>[2x]MDLKIKNKVCIITGGAKGIGYGIAKLWASEGGIPVIFSRSMPKEHDKELKKLSSEYEFYEIDLKNYEQIEKLVKKVAIKHGGIYALVNNAGTNDNLHIENTSTQDLIKSYENNLFHYYTMTKECLPYIKKEQGSILNIVSKTGITGQGRTSAYASAKAAQMGFTREWACAFAKDNVRVNAIAPAEVMTPLYEKWLQNFPNPKEQYEKIAKAIPLGHRFTTIEEIANTAVFTLSPLASHTTGQILMPDGGYVHLDRALNWDENTRGHHHHHH

We also characterize the putative dehydrogenase Cj0485 through crystallography, enzymology, and multiple biological assays to confirm its function as a fucose dehydrogenase, which we have named FucX. Several aldose sugars in both d- and l-configurations were screened as substrates and Cj0485 displayed substantial activity on l-fucose and d-arabinose and with low levels of activity on l-galactose. The Cj0485 monomer adopts a Rossmann-like fold comprising a central seven-stranded twisted β-sheet sandwiched between two trios of parallel α-helices. The holo-enzyme’s asymmetric unit contained four monomers that were arranged as tetramers with identical D2 symmetry to the crystallographic tetramer observed in the apo-complex. PISA31 analysis predicts this recurring tetramer to be a stable conformation, supporting the likelihood that the tetramer is the biologically relevant assembly of the enzyme.

To provide insight into the substrate specificity of Cj0485, we solved X-ray crystal structures of this enzyme alone and in complex with NADP+. The apo-enzyme crystallized in the space group C2221 with two monomers in the asymmetric unit and the crystallographic lattice generates a tetramer with D2 symmetry. A Cj0485 monomer from the apo-structure superimposes on an apo-FabG monomer with a root-mean-square-deviation (RMSD) of 0.9 Å (over 246 matched Cα atoms) revealing the similarity of the folds. Furthermore, the tetramer of Cj0485 superimposes on the tetramer of apo-FabG with an RMSD of 0.99 Å (over 1003 matched Cα atoms) indicating adoption of the same tetrameric organization.> SHSEEPAEILPPARDEEEEEEEGMEQGLEEEEEVDPRIQGELEKLNQSTDDINRRETELEDARQKFRSVLVEATVKLDELVKKIGKAVEDSKPYWEARRVARQAQLEAQKATQDFQRATEVLRAAKETISLAEQRL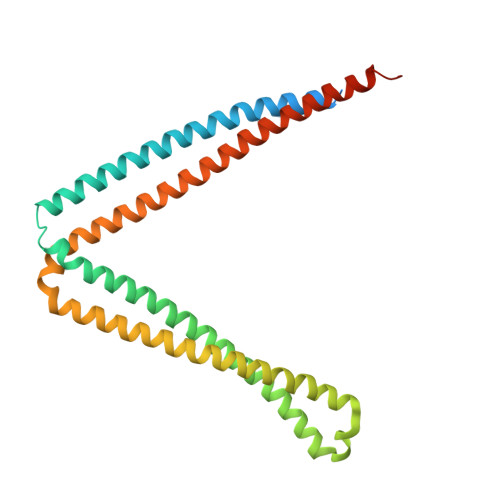LEDDKRQFDSAWQEMLNHATQRVMEAEQTKTRSELVHKETAARYNAAMGRMRQLEKKLKRAINKSKPYFELKAKYYVQLEQLKKTVDDLQAKLTLAKGEYKMALKNLEMISDEIHERRRSSAMGPRGCGVGAE Inositol polyphosphate 1-phosphatase (INPP1) is a prototype member of metal-dependent/lithium-inhibited phosphomonoesterase protein family defined by a conserved three-dimensional core structure. Enzymes within this family function in distinct pathways including inositide signaling, gluconeogenesis, and sulfur assimilation. INPP1 catalyzes the metal-dependent hydrolysis of the phosphomonoester bond from the 1 position phosphate of Ins(1,4)P2 or Ins(1,3,4)P3 to yield inositol 4-phosphate and inositol 3,4-bisphosphate, respectively. Conserved secondary structural elements comprise juxtaposed metal binding pockets and define a shared sequence pattern of D54…E79E80…D153PID156S157T158…D317 as shown for INPP1.

We therefore tested the effect lithium addition in the presence of substrate. INPP1 was co-crystallized in the presence of 10X molar excess of Ins(1,3,4)P3 and 2 mM Gd3+, but also 200 mM Li+. In the presence of substrate, no electron density peak was observed for Gd3+ at metal site GD3 with little change in density observed at metal site GD1. A 15.4σ difference density peak was found for metal site GD1, with no detectable peak for metal site GD3 indicating lithium displaces metal at site GD3 and that binding requires the presence of substrate. Interestingly, a 4.9σ difference density peak was found for gadolinium binding at GD2, the equivalent of MG2, indicating poorly ordered Gd3+ in that site. This provides further evidence Li+ does not displace metals at either sites GD1 or GD2. In dramatic contrast, co-crystallization of INPP1 with Gd3+, I(1,3,4)P3 and Li+ resulted in a stunning complete loss of electron density at metal site GD3 (no observable density even at below 1 sigma) with little change in density at site GD1 (remained above 20 sigma). Because we did not observe significant changes in the side-chain geometry for residues that coordinate the metal binding sites, we infer the parsimonious explanation is lithium replaces gadolinium at metal site 3. A partially ordered Gd3+ was found in metal site GD2 in the substrate-bound, lithium-treated structure and importantly excludes this metal site as the lithium-binding site. In the Gd3+/Ins(1,3,4)P3 and Gd3+/Li+/Ins(1,3,4)P3 structures, the ion could either be a phosphate from the Ins(1,3,4)P3 substrate molecule or a sulfate from the Gd2(SO4)3 in the crystallization solutions.

> MSDILQELLRVSEKAANIARACRQQETLFQLLIEEKKEGEKNKKFAVDFKTLADVLVQEVIKENMENKFPGLGKKIFGEESNELTNDLGEKIIMRLGPTEEETVALLSKVLNGNKLASEALAKVVHQDVFFSDPALDSVEINIPQDILGIWVDPIDSTYQYIKGSADITPNQGIFPSGLQCVTVLIGVYDIQTGVPLMGVINQPFVSQDLHTRRWKGQCYWGLSYLGTNIHSLLPPVSTRSNSEAQSQGTQNPSSEGSCRFSVVISTSEKETIKGALSHVCGERIFRAAGAGYKSLCVILGLADIYIFSEDTTFKWDSCAAHAILRAMGGGMVDLKECLERNPDTGLDLPQLVYHVGNEGAAGVDQWANKGGLIAYRSEKQLETFLSRLLQHLAPVATHT> MTVNWDINEALKNYMSDPSTIQTPEADSALVDCENDPESLLDNGLINSVLNPIVDAVAESPDAITRSHIFDSLQFLLKYTSYLSTHALSKLFDLITSGLGAEADVVHHDLESDEQELIPAHKQLLEMYGFLLQWTLTAAEAKAAEKSSTTVPARGRGKPKSKTGPGQDGTWDSVRQLETALSTMCKVLRLKLGKIFITTSERDTFIGLLTRPVYMILESEQRVKNTSIRMHAFKVLCMAVKHHGHGYAAQVSIVQNLTYFEHLSEPMAEFLHILAEQYDYPQLADEVLRELSNKEFNSNDTKGPKSVSAFMIRLSELAPRLVIKQVTLLAKQLDSESYTLRCALIEVFGNMLAYLSKSEERGENHKSQMNAFFDVLEERFLDINPYCRCRTIQVYIKLCELDQKFPKRRQRAAELACRSLMDKSSHVRRNAIKLLATLIRTHPFTALHGAQLARKDWQERLERVEAELNVLKPPPEAAGLEGDKANTSADQGLLDDATQVDSPKKRLEDMTEEEKIEAVRKAQEQAATSEAIEKLTLTKRYYTEALKFIDVLHEATPVICQLLGSKNKSEVIEAMDYFEIGDAYNIEQNKIGIRKMLRLIWTKGSSDEGKGVQTHLIECYKRLFFEAPDSFSPNDAANYIARNMISLTFGATPAELTSLEQLLHLMMKQGMIPDLVIAKLWQVYGVQRREISKKQRRGAIIVLGMLATASPEIVVGEMETMLRIGLGAHGRADLQLAKYTCIALRRINPTSRQTEKGSTTTFSRLPNDHAVLVKLAAITEVPTDNKEWYGVAEQAINAIYALSKHPDVLCSEIIRRKTRAVFARSTSKESVIGLSQLLFIVGHVAIKQIVHLELCELDFKRRKQEKDKEKAQQQEQEDNELDMIGGTTEDDFTEAMAHIRERELLFGPQSLLAQFGPMVSEICANNTVYKDRNLQQAATLCLAKLMCVSSEYCEANLPLLITIMERSPDPTVRSNAVIALGDMAVCFNHLIDENTDFLYRRLADPQPMVKRTCLMTLTFLILAGQVKVKGQLGEMAKCLEDEDKRIADLARMFFTELSTKDNAV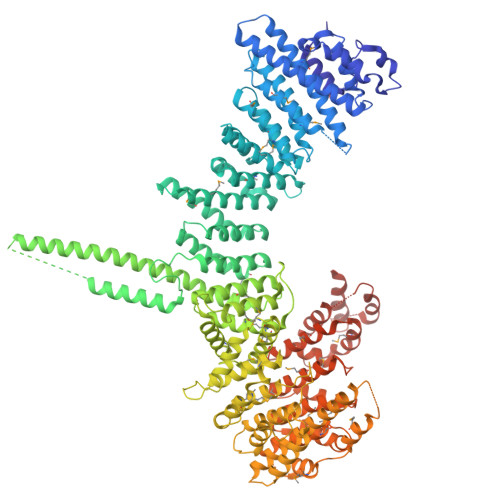YNHFVDMFSLLSADERIDEEAFRRIVRFLLGFVEKDKXXXXXXXXXXXXXXXXXXXXXXXXXXXXXXXXXXXXXXXXXXXXXXXXXXXXXX> MPEGADPVAEVKTALAGFLKEVKGFQDDVKTRLQQQEERVTMLQTKTYAGRHALAAAATEEAPHQKAFAAYLRTGDDDGLRGLSLEGKALNSAVAAEGGYLVDPQTSETIRGVLRSTASLRQIASVVNVEATSFDV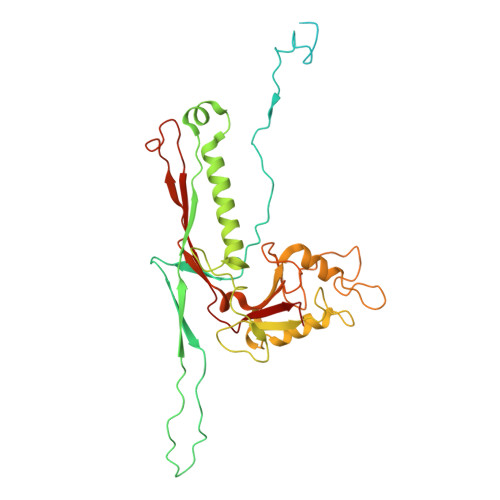LVDKTDMGSGWASETAALSETATPQIDRITIPLHELAAMPKASQRLLDDSAFDIETWLANRIADKFARAEAAAFISGDGVDKPTGFLTKTKVANGAWAWGSLGYVATGAAGDFAAVNASDAVVDLVYALGAEYRANASFVMNSKTAGAVRKMKDADGRFLWADSLAAGEPARLMGYPVLIAEDMPDIAANAYAIAFGDFGNGYTIAERPDLRVLRDPFSAKPHVLFYASKRVGGDVSDFAAIKLLKFAA>[2x]GVTLLLPEPEWTYPRLSCPGSTFQKALLISPHRFGETKGNSAPLIIREPFIACGPKECKHFALTHYAAQPGGYYNGTRGDRNKLRHLISVKLGKIPTVENSIFHMAAWSGSACHDGKEWTYIGVDGPDNNALLKIKYGEAYTDTYHSYANNILRTQESACNCIGGNCYLMITDGSASGISECRFLKIREGRIIKEIFPTGRVKHTEECTCGFASNKTIECACRDNSYTAKRPFVKLNVET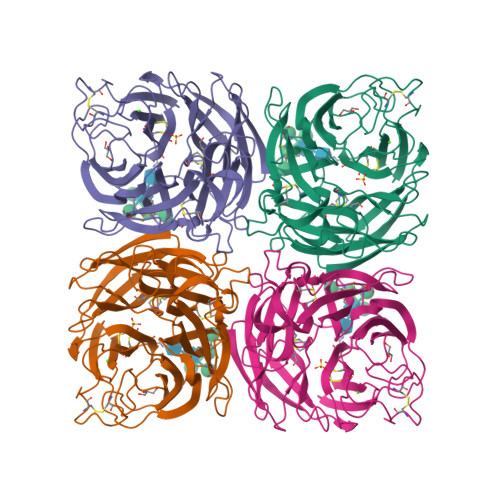DTAEIRLMCTETYLDTPRPDDGSITGPCESNGDKGSGGIKGGFVHQRMASKIGRWYSRTMSKTKRMGMGLYVKYDGDPWTDSDALALSGVMVSMEEPGWYSFGFEIKDKKCDVPCIGIEMVHDGGKETWHSAATAIYCLMGSGQLLWDTVTGVDMAL>[2x]GSPNSGTLALLLDEGSKQLPQAIIIGVKKGGTRALLEFLRVHPDVRAVGAEPHFFDRSYDKGLAWYRDLMPRTLDGQITMEKTPSYFVTREAP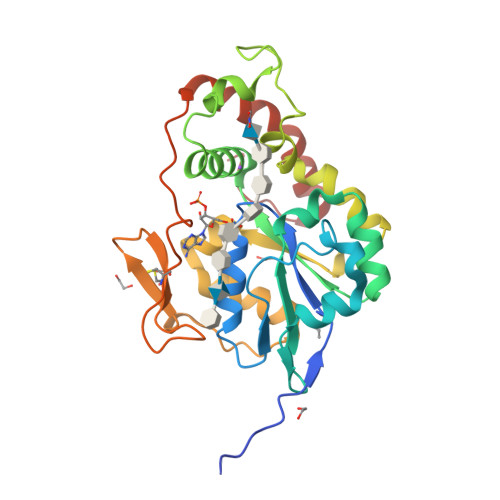ARISAMSKDTKLIVVVRDPVTRAISDYTQTLSKRPDIPTFESLTFKNRTAGLIDTSWSAIQIGIYAKHLEHWLRHFPIRQMLFVSGERLISDPAGELGRVQDFLGLKRIITDKHFYFNKTKGFPCLKKAEGSSRPHCLGKTKGRTHPEIDREVVRRLREFYRPFNLKFYQMTGHDFGWDG> ATCDDGRTTANAACCILFPILDDIQENLFDGAQCGEKVRESLRLTFHDAIGFSPTLGGGGADGSIIAFDTIETNFPANAGIDEIVSAQKPFVAKHNISAGDFIQFAGAVGVSNCPGGVRIPFFLGRPDAVAASPDHLVPEPFDSVDSILARMGDAGFSPVEVVWLLASHSIAAADKVD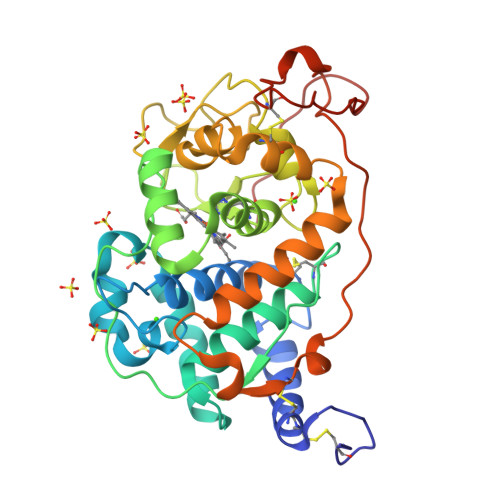PSIPGTPFDSTPGVFDSQFFIETQLKGRLFPGTADNKGEAQSPLQGEIRLQSDHLLARDPQTACEWQSMVNNQPKIQNRFAATMSKMALLGQDKTKLIDCSDVIPTPPALVGAAHLPAGFSLSDVEQACAATPFPALTADPGPVTSVPPVPRS>[4x]SHMKFTVEREHLLKPLQQVSGPLGGRPTLPILGNLLLQVADGTLSLTGTDLEMEMVARVALVQPHEPGATTVPARKFFDICRGLPEGAEIAVQLEGERMLVRSGRSRFSLSTLPAADFPNLDDWQSEVEFTLPQATMKRLIEATQFSMAHQDVRYYLNGMLFETEGEELRTVATDGHRLAVCSMPIGQSLPSHSVIVPRKGVIELMRMLDGGDN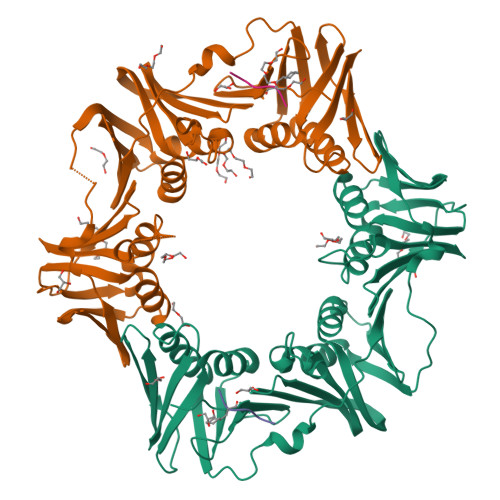PLRVQIGSNNIRAHVGDFIFTSKLVDGRFPDYRRVLPKNPDKHLEAGCDLLKQAFARAAILSNEKFRGVRLYVSENQLKITANNPEQEEAEEILDVTYSGAEMEIGFNVSYVLDVLNALKCENVRMMLTDSVSSVQIEDAASQSAAYVVMPMRL;>XQADLF[4x]N-(5-chloropyridin-2-yl)-2-oxo-2-(pyrrolidin-1-yl)acetamide | C11 H12 Cl N3 O2 | 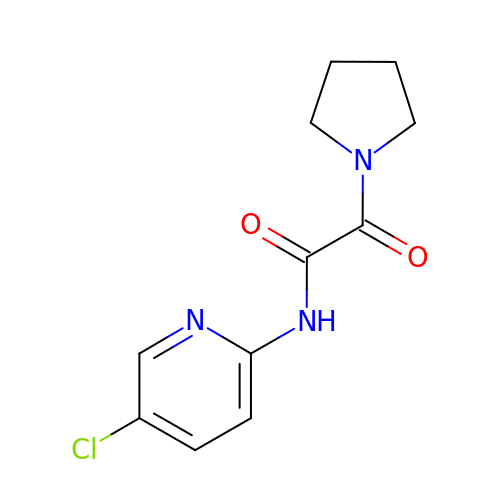LBTQVDWFWLGFOP-UHFFFAOYSA-N> GSKWKVFIDQINRSLENYEPCSSQNCSCYHGVIEEDLT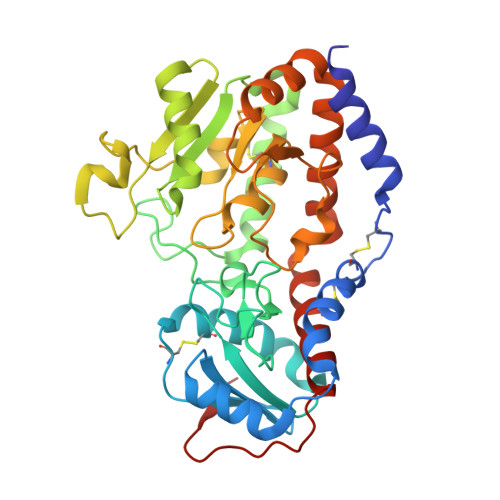PFRGGISRKMMAEVVRRKLGTHYQITKNRLYRENDCMFPSRCSGVEHFILEVIGRLPDMEMVINVRDYPQVPKWMEPAIPVFSFSKTSEYHDIMYPAWTFWEGGPAVWPIYPTGLGRWDLFREDLVRSAAQWPWKKKNSTAYFRGSRTSPERDPLILLSRKNPKLVDAEYTKNQAWKSMKDTLGKPAAKDVHLVDHCKYKYLFNFRGVAASFRFKHLFLCGSLVFHVGDEWLEFFYPQLKPWVHYIPVKTDLSNVQELLQFVKANDDVAQEIAERGSQFIRNHLQMDDITCYWENLLSEYSKFLSYNVTRRKGYDQIIP> MAKSGNYSYKRWVFTINNPTFEDYVHVLEFCTLDNCKFAIVGEEKGANGTPHLQGFLNLRSNARAA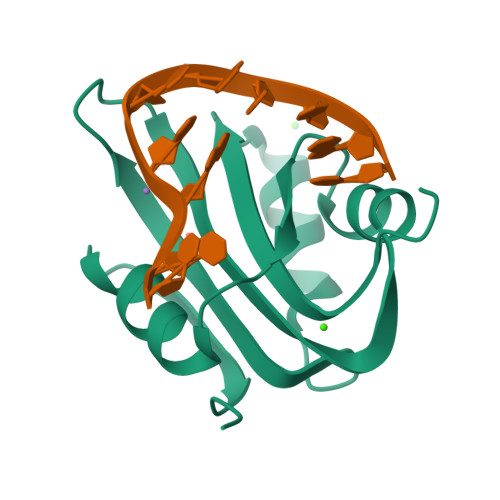ALEESLGGRAWLSRARGSDEDNEEFCAKESTYLRVGEPVSKGRSS> LKTEWPELVGKSVEEAKKVILQDKPEAQIIVLPVGTIVTMEYRIDRVRLFVDK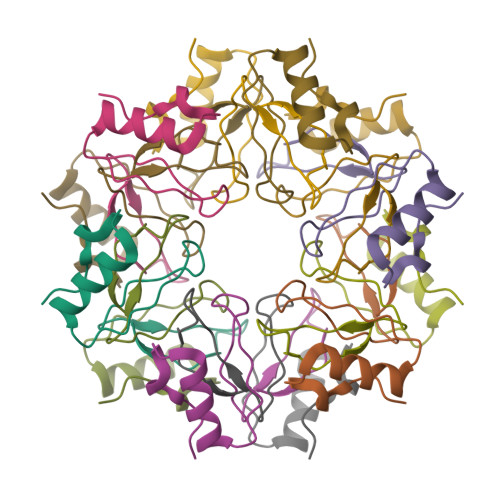LDNIAEVPRVG>MGSSHHHHHHSQDPMQASRLGELLVRNNIITKEQLAKALDEQRTSGGQQRLGSILVKNGLVTEPDLTTFLSKQYGVPSINLSEFEADMAVVKIIPADVAQKYQIVPVNRAGSTLIIAMADPSNIFAIDDIKFMTGYNVEVVVASESSIKTAIDKYYDQSASLADVMNDLEMDDLEVIGEDEDVDVSSLERATEDAPVVKLVNLILTDAIKKKASDIHIEPYERTFRVRYRIDGVLYEVMKPPLKLKNAITSRIKIMADLDIAERRLPQDGRIKIKMGGGQDMDYRVSVLPTLFGEKVVLRLLDKSNLQLDMTKLGYEPTALSYFKEAIHKPFGMVLVTGPTGSGKTVSLYSALSELNKTTENISTAEDPVEFNFAGINQVQMHEDIGLTFAAALRSFLRQDPDIIMIGEIRDFETAEIAIKAALTGHLVLSTLHTNDAPATINRLLNMGVEPFLVASAVNLITAQRL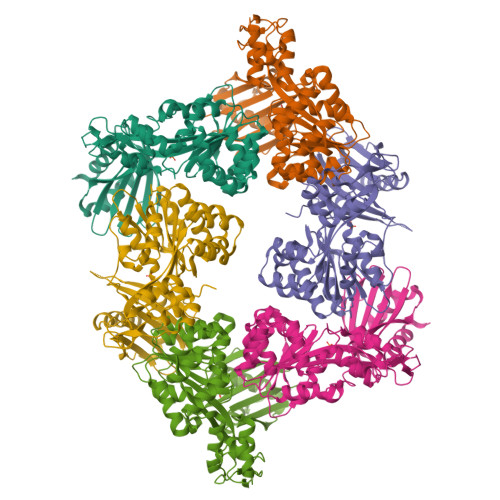ARRVCSECKAVEEIPIQALIDAGVPPEEAPEYVCFRGTGCAKCNNTGYKGRVGFYQVMPMLEEIRELILNGANTAEIKRESMRLGIKTMRQSGLTKLKEGVTSFEEVLRVTVADD[3x]2-[[[2-[2-(dimethylamino)ethyl-ethyl-amino]-2-oxidanylidene-ethyl]amino]methyl]pyridine-4-carboxamide | C15 H25 N5 O2 | 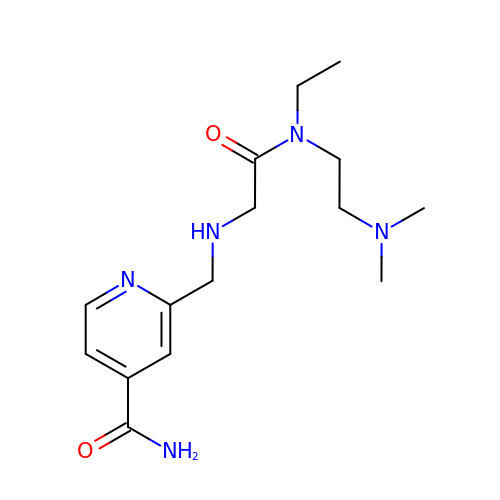PNFMVADNCOGWME-UHFFFAOYSA-N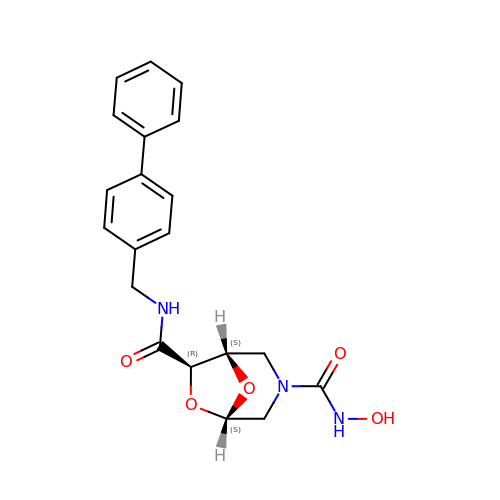(1S,5S,7R)-N~7~-(BIPHENYL-4-YLMETHYL)-N~3~-HYDROXY-6,8-DIOXA-3-AZABICYCLO[3.2.1]OCTANE-3,7-DICARBOXAMIDE | C20 H21 N3 O5 | PPLDARNGJSQINK-OKZBNKHCSA-N> MANAIRLPPEAYPMSIAAQKNDDDRQARALAALAEKPDGIVEAIAAKAEVAPAEILAILPQGAAVSAPADRFDAIWNEMRGWGEILMIVQTGDIVLEVPGHLPEGTESHGWFNIHGDSPIGGHIKKDNCAAITFVDRGFHGRRSCSVWFMNAAGGAMFKIFVRRDENKELLAGQLAKFEEL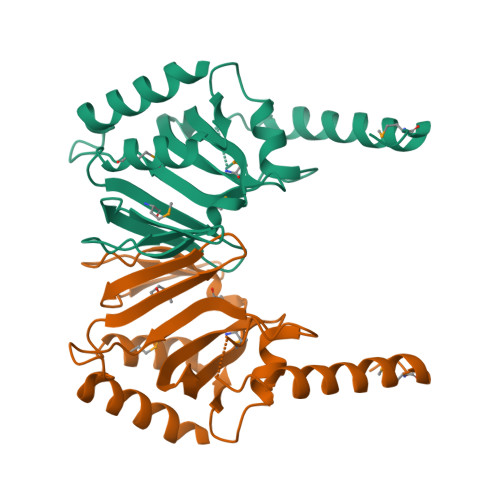RDGFRGLEHHHHHH(3R)-3,31-dimethyl-7,11,15,19,23,27-hexamethylidenedotriacont-31-en-1-yl dihydrogen phosphate | 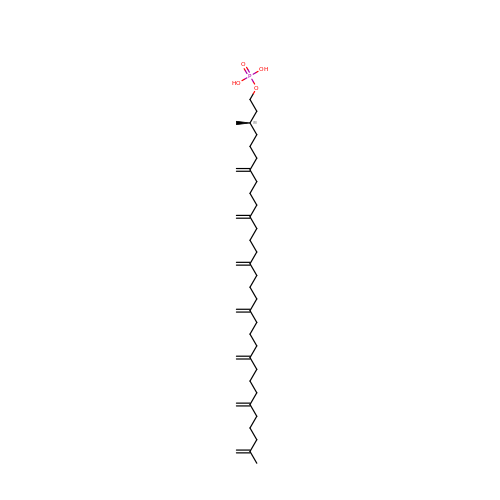C40 H69 O4 P | CTKMEBTWSXRRSJ-RRHRGVEJSA-N>[3x]ADIYPEFGTYPGGGES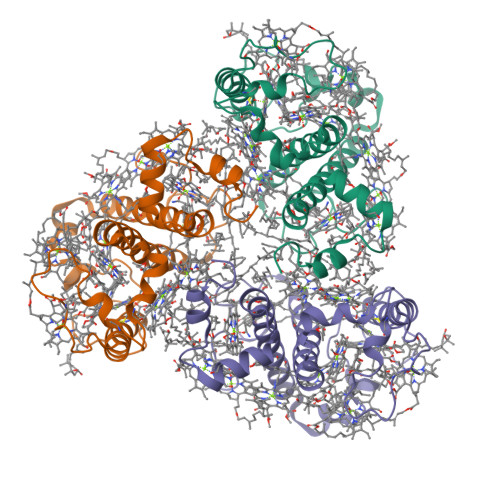PIIPFGSEKNAEREVIHGRWAMLGVTGAWAAENGTGIPWFTAGTLCTPDDCTAVADKFPGAVAPLAPEGSGYPSFWNVLIIEIVLVGAAEAYRTGISDSPFDDGLTVGDVNPGGRFDPLGLAESGDLEELKIKELKHCRLSMFAWLGCIFQALATQEGPIANWQSHVADPVHSNVLTNAAKGFGFY> A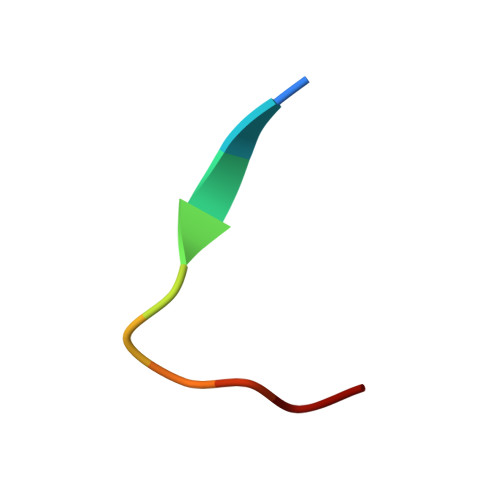KTIKITQTR> MGPDEPERPALLILELKSYARGVRVADAALKAAPVRLLKCKIVEPGKALIMLTGR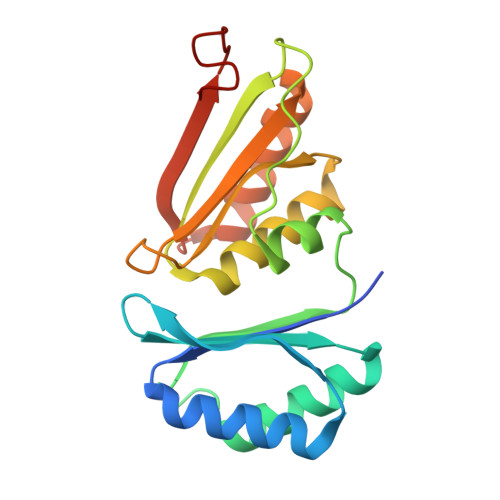PEDVEKAYKAALTVANKGSGNLIDSVFIPAIHPALLPFLLEETPAPPLEDPDRALLFVEVKTVAAAIRAADAALRAAPVELVRMRLSEHIGGKAVFALVGDPADVLRAAAVVAEVAGDQLLDIAIIPRPHPALLGREFF> HMVPMDKTLKEFGADVQWDDYAQLFTLIKDGAYVKVKPGAQTAIVNGQPLALQVPVVMKDNKAWVSDTFINDVFQSGLDQTFQVEKRPHPLNALTADEIKQAVEI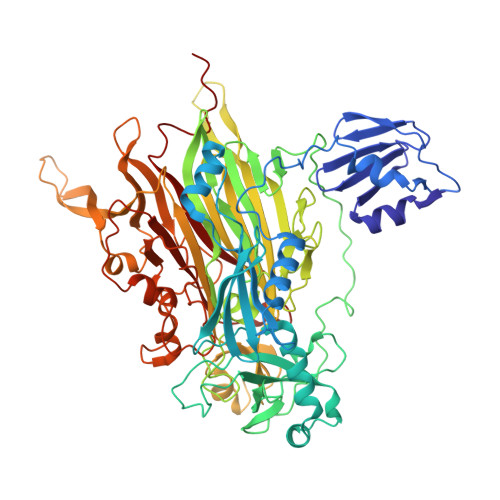VKASADFKPNTRFTEISLLPPDKEAVWAFALENKPVDQPRKADVIMLDGKHIIEAVVDLQNNKLLSWQPIKDAHGMVLLDDFASVQNIINNSEEFAAAVKKRGITDAKKVITTPLTVGYFDGKDGLKQDARLLKVISYLDVGDGNYWAHPIENLVAVVDLEQKKIVKIEEGPVVPVPMTARPFDGRDRVAPAVKPMQIIEPEGKNYTITGDMIHWRNWDFHLSMNSRVGPMFSTVTYNDNGTKRKVMYEGSLGGMIVPYGDPDIGWYFKAYLDSGDYGMGTLTSPIARGKDAPSNAVLLNETIADYTGVPMEIPRAIAVFERYAGPEYKHQEMGQPNVSTERRELVVRWISTVGNYDYIFDWIFHENGTIGIDAGATGIEAVKGVKAKTMHDETAKDDTRYGTLIDHNIVGTTHQHIYNFRLDLDVDGENNSLVAMDPVVKPNTAGGPRTSTMQVNQYNIGNQQDAAQKFDPGTIRLLSNPNKENRMGNPVSYQIIPYAGGTHPVAKGAQFAPDEWIYHRLSFMDKQLWVTRYHPGERFPEGKYPNRSTHDTGLGQYSKDNESLDNTDAVVWMTTGTTHVARAEEWPIMPTEWVHTLLKPWNFFDETPTLGALKK~{N}-[(1-azanylcyclohexyl)methyl]-1-methyl-6-oxidanylidene-pyridine-3-carboxamide | C14 H21 N3 O2 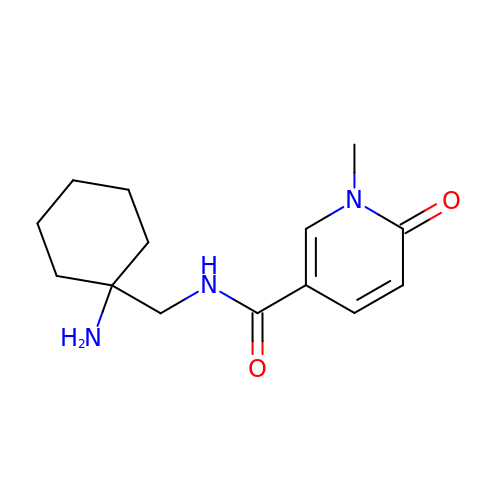| OYMFRGAWSOVJKP-UHFFFAOYSA-N> GGTDINKLIEEGKKHYLPKTYTFDNGKIIIKAGDKVEESKIQKLYWASKEVKSQFHRIIGNDKPLEVGNADDILTIVIYNNPEEYKLNKTLYGYSVDNGGIYIEGIGTFFTYERTPQESIYSLEELFRHEFTHYLQGRYLIPGLFN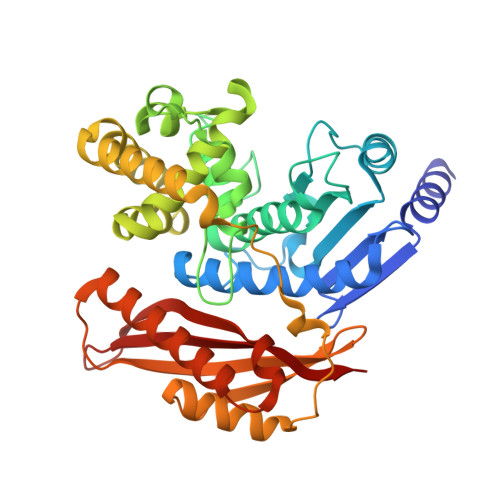KGDFYKGNNGRITWFEEGSAEFFAGSTRTSVLPRKSMVGGLSKNPKERFNADKLLHSKYSDGWDFYKYGYAFSDYMYNNNKKLFSDLVSTMKNNDVKGYEALIEESSKDSKINKDYEYHMENLVNNYDNYTIPLVSDDYMKQYDNKSLHEIKSDIEKAMDVKNSQITKESSQYFDTYNLKATYTLSSNKGEISNWNYMNNKINEALNKLDNLSWGGYKTVTAYFSNPRLNSNNEVVYDIVFHGLLSHN>QDADKLPHTKVTLVAPPQVHPHEQATKSGPKVVEFTMTIEEKKMVIDDKGTTLQAMTFNGSMPGPTLVVHEGDYVQLTLVNPATNAMPHSVDFHGATGALGGAKLTNVNPGEQATLRFKADRSGTFVYHCAPEGMVPWHVVSGMSGTLMVLPRDGLKDPQGKPLHYDRAYTIGEFDLYIPKGPDGKYKDYATLAESYGDTVQVMRTLTPSHIVFNGKVGALTGANALTAKVGETVLLIHSQANRDTRPHLIGGHGDWVWETGKFANPPQ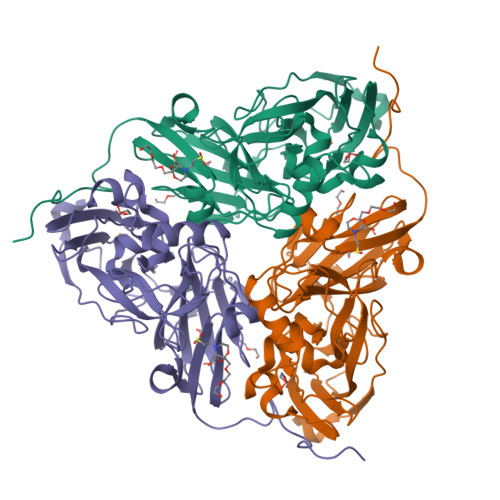RDLETWFIRGGSAGAALYTFKQPGVYAYLNHNLIEAFELGAAGHIKVEGKWNDDLMKQIKAPAPIPR[2x]> VVRVADTMPSGPSNSESIPALTAAETGHTSQVVPSDTIQTRHVRNFHVRSESSVENFLSRSACVYIVEYKTRDDTPDKMYDSWVINTRQVAQLRRKLEFFTYVRFDVEVTFVITSVQD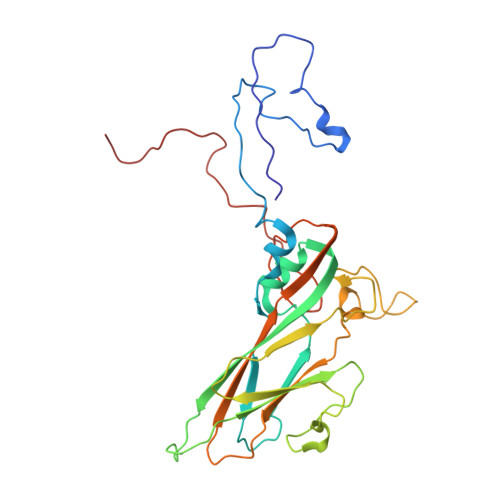DSTRQNTDTPALTHQIMYVPPGGPIPQAVDDYNWQTSTNPSVFWTEGNAPPRMSIPFMSVGNAYSNFYDGWSHFSQTGVYGFNTLNNMGKLYFRHVNDKTISPITSKVRIYFKPKHVKAWVPRPPRLCEYTHKDNVDFEPKGVTTSRTQLTISNSTHVEN>GHMSQEEKLPKILIVEDDERLARLTQEYLIRNGLEVGVETDGNRAIRRIISEQPDLVVLDVMLPGADGLTVCREVRPHYHQPILMLTARTEDMDQVLGLEMGADDYVAKPVQPRVLLARIRALLRRTDKTVE[2x]

BfmR is the response regulator of a two-component signal transduction system (TCS) which propagates the signal from its corresponding sensor histidine kinase BfmS and acts as a transcriptional regulator. The OmpR/PhoB family of response regulators is activated by autophosphorylation of a conserved aspartate residue in the receiver domain (Asp58 in BfmR). Phosphorylation induces an equilibrium shift favoring the active conformation, which includes formation of a 2-fold symmetrical homodimer involving the α4-β5-α5 face of the receiver domain. This homodimeric conformation facilitates the effector domain to bind DNA and modulate transcription.

The crystal structure of the receiver domain of BfmR was determined, lending insight into putative ligand binding sites. The space group was determined to be P65, with symmetry-related reflections scaling much poorer in the higher-symmetry P6522 space group (Rmerge, 8.6% versus 35.2%, respectively, to 2.10-Å resolution). The final refined model possessed a defining electron density for Lys6-Thr125 for both protomers, plus 181 modeled solvent molecules. Moreover, the divalent cation (Mg2+ or Mn2+) required for autophosphorylation was not observed in the electron density in the cleft neighboring Asp58. A search of the PDB revealed that this specific homodimer interface has not been previously observed for response regulator receiver domains. Predicted binding hot spots exist at the homodimer interface and the phosphorylation site.>[2x]GSDYIIKEKTVLLQKKDSEGFGFVLRGAKAQTPIEEFTPTPAFPALQYLESVDEGGVAWRAG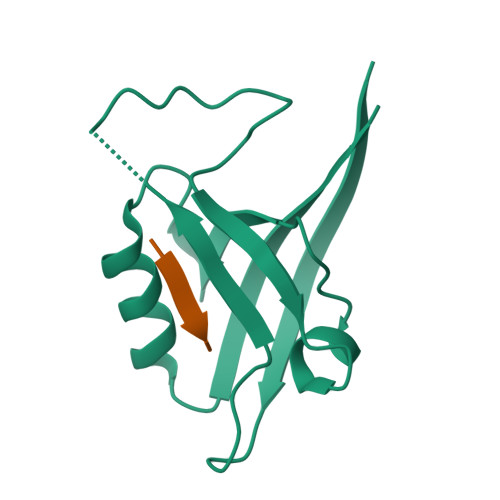LRMGDFLIEVNGQNVVKVGHRQVVNMIRQGGNTLMVKVVMVTRHPDMDEAVHK;>DETNL[2x]> MHHHHHHAVRASEISRVYEAYPEKKATLYFLVLGFLALIVGSLFGPFQALNYGNVDAYPLLKRLLPFVQSYYQGLTLHGVLNAIVFTQLFAQAIMVYLPARELNMRPNMGLMWLSWWMAFIGLVVAALPLLANEATVLFTFYPPLKGHWAFYLGASVFVLSTWVSIYIVLDLWRRWKAANPGKVTPLVTYMAVVFWLMWFLASLGLVLEAVLFLLPWSFGLVEGVDPLVARTLFWWTGHPIVYFWLLPAYAIIYTILPKQAGGKLVSDPMARLAFLLFLLLSTPVGFHHQFADPGIDPTWKMIHSVLTLFVAVPSLMTAFTVAASLEFAGRLRGGRGLFGWIRALPWDNPAFVAPVLGLLGFIPGGAGGIVNASFTLDYVVHNTAWVPGHFHLQVASLVTLTAMGSLYWLLPNLTGKPISDAQRRLGLAVVWLWFLGMMIMAVGLHWAGLLNVPRRAYIAQVPDAYPHAAVPMVFNVLAGIVLLVALLLFIYGLFSVLLSRE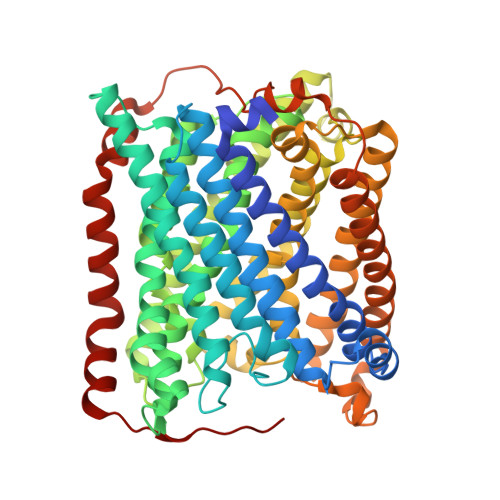RKPELAEAPLPFAEVISGPEDRRLVLAMDRIGFWFAVAAILVVLAYGPTLVQLFGHLNPVPGWRLW> DLALSCGTSEASADQDKKKWEPDTKFLKTGNSIHATATYQDPSLLSTVPYMTARIFTAPATYEIPIKGDKRHLLRLYFYPSTYTGLNISNSYFTVEANDVTLLSNFSAAITCQALTQAYLVKEYSLAPTDKDVLSIKFTPSDKYRDAFAFINGIEVIQMPELFDTAALVGFTDQTMDAKTANLQSMFRLNVGGQDIPGSQDSGGLTRTWYNDAPYIFSAGLGVTLQASNNFRINYQNMPVSIAPADIYKTARSQGPNGDINLKSNLTWMFQIDKNFTYILRL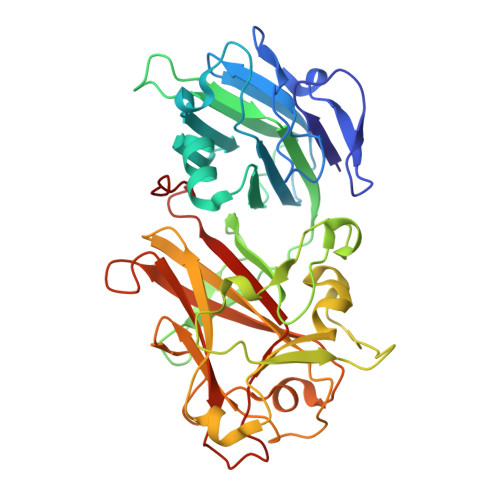HFCEFQLSKINQKVFNIYINNRTAQADTTPADIIGWTGEKGIPMYKDYAIYVDANNGGEEITLQMTPSTFGQPEYYDSSLNGLEIFKMDTMKNLAGPNPEP> SMENILNDINKRFISLPEEDVRGNKQILESVLRTFVEQMKTQDPLFKALFRRVFYGGSFYDGLKVGKPEEFDLDILLHIPIYAQPVLNESNVPGFVWLKLNNLDGWLRQPEGRVYKDFRKKFLADNDFLDTGKTLRWMESLVQKTLNTLPWVNNATCELTNEFGTFHINWWKGGPAMTLGISHSSGEKIMDVDLVACFVFSGDKWPINGYRSNPFPSTKPEFFIVPKKPQGPVNPQGRYWSLSFQEQERVLIDNKNRLKPAVKLIKKLKEKTHPNIASYYIKTVFLHIIEQKDQSFWNKSLREVFMTTLREYNEFIADQSIPYYWCRKNNLIGHLAPITLNNISNRIGYIIKDIENNPENIAKHLLTKEEYTKYIQGEDVMAEALPALPASQTSSCVII

Cyclic GMP–AMP synthase (cGAS) is a cytosolic DNA sensor that produces the second messenger cG[2′–5′]pA[3′–5′]p (2′3′-cGAMP) and controls activation of innate immunity in mammalian cells. Here we show that cGAS-like receptors (cGLRs) are innate immune sensors that are capable of recognizing divergent molecular patterns and catalysing synthesis of distinct nucleotide second messenger signals. In support of this conclusion, Hartmann, Imler, Cai and colleagues have identified cGLR2 as a second functional cGLR in Drosophila and have demonstrated in vivo that cGLR1 and cGLR2 have discrete roles in Drosophila immunity. Together, our results define cGLRs as receptors in animal cells that are capable of detecting diverse pathogen-associated molecular patterns and dictating response to the foreign environment.

To define the function of cGAS-like enzymes in animals, we screened predicted cGAS homologues for suitability in structural analysis and determined a 2.4 Å crystal structure of the human protein MB21D2 (hMB21D2; encoded by C3orf59) and a 1.6 Å crystal structure of a protein from the beetle species Tribolium castaneum (GenBank XP_969398.1). Despite divergence in the primary sequence, the hMB21D2 and T. castaneum XP_969398.1 structures each reveal close homology to human cGAS with a shared bi-lobed architecture, a caged nucleotidyltransferase core, a Gly-[Gly/Ser] activation loop and a putative catalytic triad. A conserved groove is present in both the hMB21D2 and the T. castaneum XP_969398.1 structures, but is notably distinguished by the absence of a Zn-ribbon and the insertion of a C-terminal α-helix in hMB21D2. In contrast to hMB21D2, the surface of T. castaneum XP_969398.1 shares highly conserved basic residues with human cGAS and we therefore tested this enzyme with candidate DNA and RNA ligands. We observed that T. castaneum XP_969398.1 is activated to synthesize a nucleotide product upon recognition of double-stranded RNA (dsRNA).> MGIISYVKKLFKRPAGEIMRMSSGNIGVYKLDDSRVDYELARELYQNKNANYKLGSSFVRPIVNSTTGFMGVPHFQIEDEEAQYILDEFVLDNTSKMLKTHTDSLKQGDCYIWITREERENPLYPDKKVRL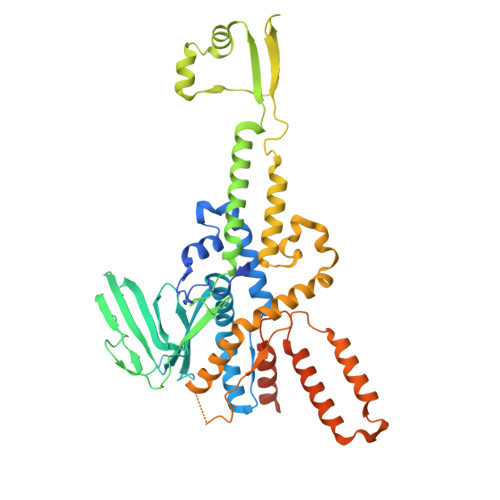IYNFISPEEVKEIILDPTTKEPIAYILESQNEWTDLGENKRKAKVKQIITAESRFVEVEGDKIEGLEEGETPNVWGFIPIIHFKNEADETLKYGQSDIEPIEPLLKAYHDVMLHALKGSKMHSTPKLKLKLTDVASFLAHNFGVEDPVKFAKEGGKINLDGHEILFLNKDEEAEFVEVKSAIGDAKELLKLLFYCIVDVSETPEFIFGVHTPSALASVKEQMPIMVNKIRRKREQFTNSWQLLARMVLIMSSNSSGMKYSSYDVTIGWDEVNPRDDKELAETLEKVCCALDKALEGGFISEESTVNFLAQYIDTMSNYISDDGEREGEREKIIKTKMLKYRLDDSQGLNDESNEIEKEINKIKDNNGNG> GSHMQDPEQLKHCNGILKELLSKKHAAYAWPFYKPVDASALGLHDYHDIIKHPMDLSTVKRKMENRDYRDAQEFAADVRLMFSNCYEYNPPDHDVVAMARKLQDVFE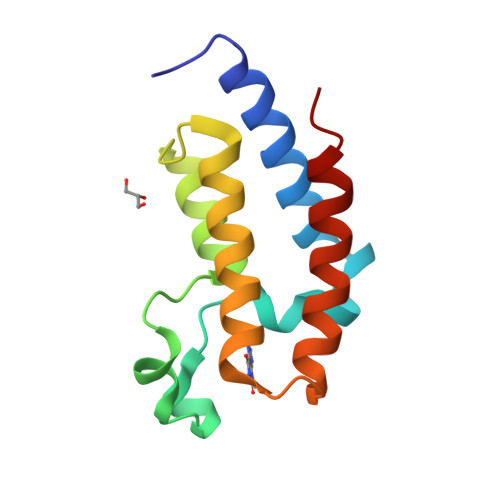FRYAKMPD POU-family transcription factors regulate metazoan gene expression via a bipartite DNA-binding domain consisting of two covalently linked helix-turn-helix subdomains, POUS and POUH. POU factors bind as dimers to DNA half-sites to form complexes with a variable quaternary structure. The POU domain combines two helix-turn-helix motifs, a tetra-helical POU-specific subdomain (POUS) and a triple-helical homeodomain (POUH)7 via a linker. OCT2 belongs to Class II of the POU family, which includes OCT1, another archetypal POU factor, and PLA1.

We solved a cocrystal structure of OCT2 bound to an optimized palindromic sequence, 5′-ATGCATATGCAT-3′ known as MORE (“More palindromic Oct factor Recognition Element”),21 which is also a functionally important POU-binding motif in chromatin. The cocrystal structure revealed nonequivalence in the subunits of the OCT2 homodimer, consistent with topologic heterogeneity of the POUX subunits. Despite the dyad symmetry in MORE, however, the asymmetric unit consisted of the OCT2 homodimer bound with the full sequence containing the two inverted octamers, in contrast with the monomer/single octamer seen in asymmetric units of the MORE-bound cocrystals of OCT1,14 Oct6,24 and Brn2.25 The resolved portions of the two OCT2 subunits aligned albeit incompletely with each other and are in good general agreement with their counterparts in the OCT1, Oct6, and Brn2 structures. The DNA termini were also nonequivalent, with one terminus in Watson–Crick base pairing but the other frayed. Nevertheless, the trajectory of the DNA in the OCT2/DNA structure fitted the 2-fold crystallographic symmetry in the other MORE-bound structures. For one POUS subdomain, the closest POUH subdomain was the one in the asymmetric unit, although it was also only ∼5 Å farther from an equivalent POUH subdomain in an adjacent unit. In contrast, the other POUS subdomain was located >10 Å closer to a POUH subdomain in an adjacent asymmetric unit. A model based on nearest neighbors would assign one pair of POUX subdomains axially along the DNA within the same asymmetric unit, as in other MORE-bound structures, while placing the other subunit in a cross-link across adjacent asymmetric units. As OCT2 carries the longest linker among POU factors, other combinations not limited by linker length are also possible. The evidence therefore suggested that the OCT2 adopted mixed linker topologies in the OCT2/MORE crystal lattice.

>[4x]GSHMEEPSDLEELEQFARTFKQRRIKLGFTQGDVGLAMGKLYGNDFSQTTISRFEALNLSFKNMCKLKPLLEKWLNDAETMSVDSSLPSPNQLSSPSLGFDGLPGRRRKKRTSIETNVRFALEKSFLANQKPTSEEILLIAEQLHMEKEVIRVWFCNRRQKEKRINP> MHHHHHHSSGRENLYFQGMAPSTPLLTVRGSEGLYMVNGPPHFTESTVFPRESGKNCKVCIFSKDGTLFAWGNGEK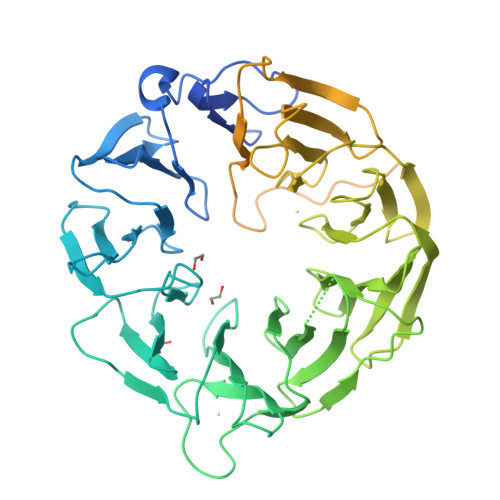VNIISVTNKGLLHSFDLLKAVCLEFSPKNTVLATWQPYTTSKDGTAGIPNLQLYDVKTGTCLKSFIQKKMQNWCPSWSEDETLCARNVNNEVHFFENNNFNTIANKLHLQKINDFVLSPGPQPYKVAVYVPGSKGAPSFVRLYQYPNFAGPHAALANKSFFKADKVTMLWNKKATAVLVIASTDVDKTGASYYGEQTLHYIATNGESAVVQLPKNGPIYDVVWNSSSTEFCAVYGFMPAKATIFNLKCDPVFDFGTGPRNAAYYSPHGHILVLAGFGNLRGQMEVWDVKNYKLISKPVASDSTYFAWCPDGEHILTATCAPRLRVNNGYKIWHYTGSILHKYDVPSNAELWQVSWQPFLDGIFPAKTITYQAVPSEVPNEEPKVATAYRPPALRNKPITNSKLHEEEPPQNMKPQSGNDKPLSKTALKNQRKHEAKKAAKQEARSDKSPDLAPTPAPQSTPRNTVSQSISGDPEIDKKIKNLKKKLKAIEQLKEQAATGKQLEKNQLEKIQKETALLQELEDLELGI> NQPYRTGFHFQPPKNWMNDPNGPMIYKGIYHLFYQWNPKGAVWGNIVWAHSTSTDLINWDPHPPAIFPSAPFDINGCWSGSATILPNGKPVILYTGIDPKNQQVQNIAEPKNLSDPYLREWKKSPLNPLMAPDAVNGINASSFRDPTTAWLGQDKKWRVIIGSKIHRRGLAITYTSKDFLKWEKSPEPLHYDDGSGMWACPDFFPVTRFGSNGVETSSFGEPNEILKHVLKISLDDTKHDYYTIGTYDRVKDKFVPDNGFKMDGTAPRYDYGKYYASKTFFDSAKNRRILWGWTNESSSVEDDVEKGWSGIQTIPRKIWLDRSGKQLIQWPVREVERLRTKQVKNLRNKVLKSGSRLEVYGVTAAQADVEVLFKVRDLEKADVIEPSWTDPQLICSKMNVSVKSGLGPFGLMVLASKNLEEYTSVYFRIFKARQNSNKYVVLMCSDQSRSSLKEDNDKTTYGAFVDINPHQPLSLRALIDHSVVESFGGKGRACITSRVYPKLAIGKSSHLFA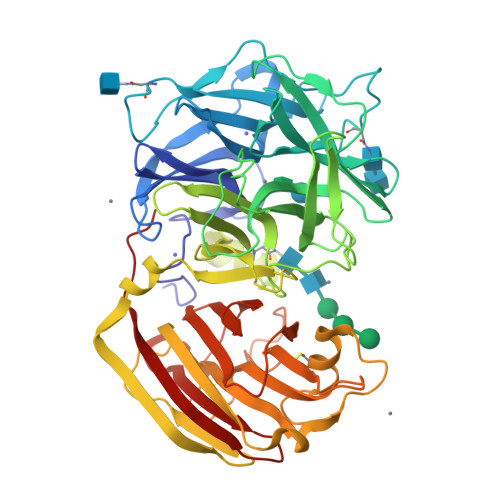FNYGYQSVDVLNLNAWSMNSAQIS> SGVIKPDMKIKLKMEGNVNGYAFVIEGEGEGKPYDGTNTINLEVKEGAPLPFSYDILTTAFAYGNRAFTKYPDDIPNYFKQSFPEGYSWERTMTFEDKGIVKVKSDISLEEDSFIYEIYLKGENFPPNGPVMQKKTTGWDASTERMYVRDGVLKGDVKHKLLLEGGGYYRVDFKTIYRAKKAVKLPDYHFVDHRIECLNHDKDHNKVTVYESAV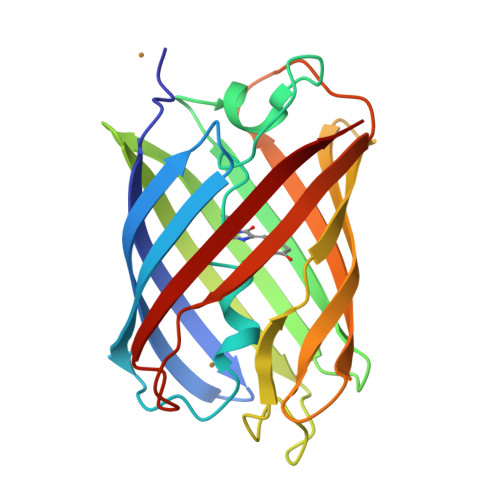ARN>[2x]GSHMRSRRVDVMDVMNRLILAM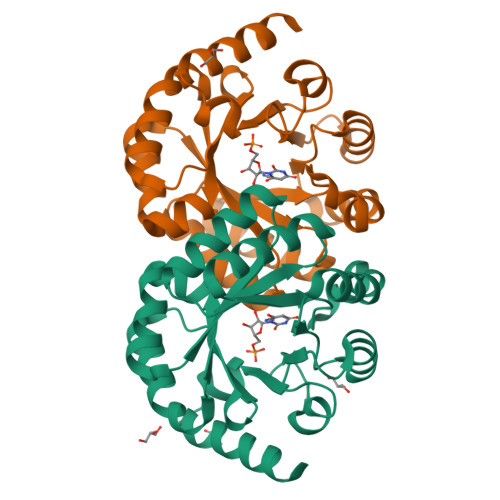DLMNRDDALRVTGEVREYIDTVKIGYPLVLSEGMDIIAEFRKRFGCRIIADFKVADIPETNEKICRATFKAGADAIIVHGFPGADSVRACLNVAEEMGREVFLLTEMSHPGAEMFIQGAADEIARMGVDLGVKNYVGPSTRPERLSRLREIIGQDSFLISPGVGAQGGDPGETLRFADAIIVGRSIYLADNPAAAAAGIIESIKDLRIPEDPAANKARKEAELAAATAEQ> MALIGQTLPSLLDIYNRTDKNGRIARIVEQLAKTNDILTDAIYVPCNDGSKHKTTIRAGIPEPVWRRYNQGVQPTKTQTVPVTDTTGMLYDLGFVDKALADRSNNAAAFRVSENMGKLQGFNNKVARYSIYGNTDAEPEAFMGLAPRFNTLSTSKAASAENVFSAGGSGSTNTSIWFMSWGE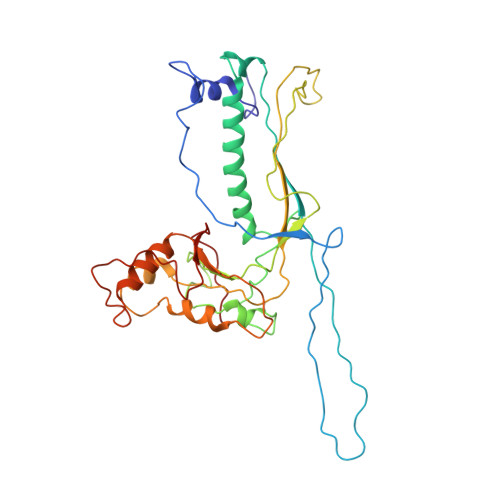NTAHMIYPEGMVAGFQHEDLGDDLVSDGNGGQFRAYRDEFKWDIGLSVRDWRSISRICNIDVTTLTKDASTGADLISMMVDAYYARDVAMLGDGKEVIYANKTIHAWLHKQAMNAKNVNLTIEEYGGKKIVSFLGIPIRRVDAILNTESAVTA> MVLFTRCEKARKEKLAAGYKPLVDYLIDCDTPTFLERIEAIQEWDRSRDDLYVWIPILDRMDGLLLKVAEKYKYKQDPKKECEVKLVEMEAHDVDYCLKMLKFTRRLLLNTENRFVYSSGDVLMYLLNCPNFTIKLAVMRILAILGERFVIAREKIVAHNIFGDHNLRKKTLKLALSLSSSVMDEDGEHFSLVDLYFDKKKVPQKWRKLRFTHYTSNDFKKSSQQKNNINETQTSIKKVTMTTQELCEHSLQQIFDKGMALLPAESWFDFSIKASVAKAFSDDSGENIDLRNIIIETKLNAIAFVNTIFSPPQVSSKLFELDPYAFNSLTDLISLSETKIPKELRTDALFTLECISLKHVWCSDIIRNLGGNISHGLLFQILRYIAKTLREATDEIDEEYNVRFFYLISNLADVKPLHESLFAAGLIPTLLEIVSIRNCPYKRTLASATHLLETFIDNSETTTEFIENDGFTMLITSVANEIDFTLAHPETWQPPKYSVVYYSISFRELAYIRSLLKLVLKLLSTDSGDRIRNLIDSPILVSLKKILENKLVFGLTLITYTLDVVQKVINSEPTIYPVLVEAGLIPYVIDNFPKLIGPSAELLSLLPDVVSAICLNPEGLKQVKEKGLINNLFDFLLDADHARILTGGDRSTEYGTDIDELARHYPDLKANIVEALCNVIRKMPSTFRNEREFLFTSPKDQKYFFHRKNEEILTDKEEHEPAYWELLDKGTMLDTFTSVLFGMSLGNGSFSQVPQHLEARDFLAIIFMENPPYEYFTSVAISNVTEVLQYLDEKYEDYAFMDVMKVLNDQLENLNDFLNSPNDRSFFLERDGENSVRSCHSKLCRLAAILNIVTNVYIDLTTLSCKRIMQIYSYFDKRGFSLIKNLKLLFQKCALEEMYIRQHMPDSVITETMPLPIVDVSGDGPPLQIYIDDPKKGDQKGKITSVKTRNTLQMRTILYTLQSNTAILFRCFLRLSHSRNMDLEHKDLTTEVHIFENVVENVIEMLKATELEGHLPYILVLLNFNTFVFTIPKASPNSTEILQTIPAYIFYQKGGYLLYLHIIRDLFTRMTKIKDLSSLDNINYIDESNGILTLSCLINALTFYNKSMQTETMENVQSIGKYYVSIDDDYNIMKALTVPIKVMALAMILDLDKSDSLFKTQSRNVPYSVFKQLLSMLKNIFTNVNIYTKELYELHWDLIFPPIKKISLFEQVGIPGDVAANYLTDTGDDLPADNSIGLFSPEQWEKYKKLIGEDKSIYYPQPMQAQYYKGCSSKELDELRDTFFNDGLPSRIFTVLPFYPKLVNAFAKTLLQIFTKYDEPTEVFAGRILDRILETDLDDPATLSSLIHLFGIFLNEKYIYQKASHLMQRFIEYLEKSLKPEHVNTPWFSKALYVYEIILAKSELPHLEELSKDVLLRYPLLSMAKVFRIPDPMKQKLFDILIRVSDISNFYSALATSRILIFYSRDELYANNIARSGILSRLLKVIGSFQKLDKINFLESSFLLLTRRCFETTENVDALIRAEINRSFTARPLGGGDDAVRELTTILEEKAHVVMRSPSQFIDVLCETARFHEFDDQGALVDYSLKRFLGEKDKNTQASSTEKSDIYERTGIMHLLLSQLMAASEKDWLSEPANSSDLPENKKAQLDPSRNPVCAYMIFLLKLLVELVSSYNQCKFEFLTFSRRNTYAERPRPRTTAINFFLYRLLDKPVGTDHDKHEAKRREVIGMLARSVIIGFLATVQDDRTTKTDVKLADPHMNFIRKFAIEAIIKAIRNATSSSKLLESNHLKLDMWFRIITSMVYVQAPYLRQLLDSNKVEADQYQLCKLVIDLGLPSVITEAMASIDLNYPFSKKIFNVAVEALNTISSTRNNFSEHFKIEDHDEVEDEVDESDKEEIPDMFKNSALGMYDVEDIEEDDDDDTSLIGDDDAMAFVDSDNGFEVVFSDEDDDMGEEDADDARSDSEENELSSEMQSSTADGTDVDYEVDDADGLIINIDQPSGDDEEMADYDANISHSSHSENEDDASMDVIEVYDDELSSGYDVDLSDYDVDESDWDSGLSSLSISDEDSESSEDEPINSTRMGDSRRRWLIAEGVELTDDSQGESEEDDRGVFRGIEHIFSNENEPLFRVHDEMRHRNHHRSINRTHFHSAMSAPSLSLLNRGRRNQSNLINPLGPTGLEQVENDISDQVTVAGSGSRPRSHHLHFSEVLVSGSFFDEPV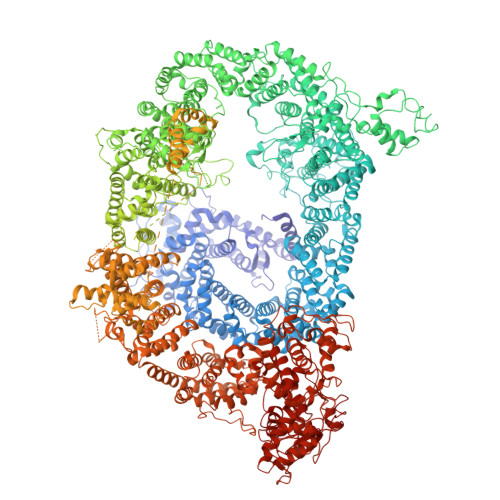LDGIILKSTVSRWKDIFDMFYDSKTYANCIIPTVINRLYKVSLALQKDLENKREQEKLKNKNLLFNEAKVESHNSSDAISVEQDDIQESNVTHDDHEPVYVTIQGSEVDIGGTDIDPEFMNALPDDIRADVFAQHVRERRAEARLNSDHNVHSREIDSDFLEAIPEDIREGILDTEAEEQRMFGRIGSSADVIRADDDVSNNDEEVENGLDHGNSNDRNNADPEKKKPARIYFAPLIDRAGIASLMKSVFISKPYIQREIYHELFYRLCSSKQNRNDLMNTFLFILSEGIIDQHSLEKVYNIISSRAMGHAKTTTVRQLPSDCTPLTVANQTIEILQSLIDADSRLKYFLIAEHDNLIVNKANNKSRKEALPDKKLRWPLWHLFSLLDRKLITDESVLMDLLTRILQVCTKTLAVLSTSSNGKENLSKKFHLPSFDEDDLMKILSIIMLDSCTTRVFQQTLNIIYNLSKLQGCMSIFTKHLVSLAISIMSKLKSALDGLSREVGTITTGMEINSELLQKFTLPSSDQAKLLKILTTVDFLYTHKRKEEERNVKDLQSLYDKMNGGPVWSSLSECLSQFEKSQAINTSATILLPLIESLMVVCRRSDLSQNRNTAVKYEDAKLLDFSKTRVENLFFPFTDAHKKLLNQMIRSNPKLMSGPFALLVKNPKVLDFDNKRYFFNAKLKSDNQERPKLPITVRREQVFLDSYRALFFKTNDEIKNSKLEITFKGESGVDAGGVTREWYQVLSRQMFNPDYALFLPVPSDKTTFHPNRTSGINPEHLSFFKFIGMIIGKAIRDQCFLDCHFSREVYKNILGRPVSLKDMESLDPDYYKSLVWILENDITDIIEETFSVETDDYGEHKVINLIEGGKDIIVTEANKQDYVKKVVEYKLQTSVKEQMDNFLVGFYALISKDLITIFDEQELELLISGLPDIDVDDWKNNTTYVNYTATCKEVSYFWRAVRSFDAEERAKLLQFVTGTSKVPLNGFKELSGVNGVCKFSIHRDFGSSERLPSSHTCFNQLNLPPYESYETLRGSLLLAINEGHEGFGLALEVLFQGP> GSGGGDDMSNAGDFLNDNAVEIPSFSKGIINDDEDDEDLMMASGRPRQRSHILEDDENSVDISMLKTGSSLLKEEEEDGQEGSIHNLPLVTSQRPFYDGPMPTPRQKPFQSGSTPLHLTHRFMVWNSIGIIRCYNDEQDNAIDVEFHDTSIHHATHLSNTLNYTIADLSHEAILLACESTDELASKLHCLHFSSWDSSKEWIIDLPQNEDIEAICLGQGWAAAATSALLLRLFTIGGVQKEVFSLAGPVVSMAGHGE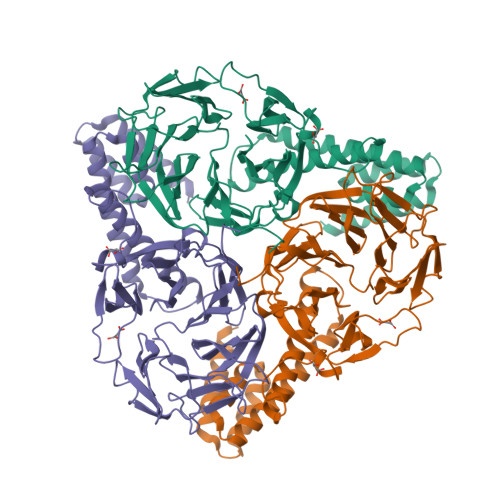QLFIVYHRGTGFDGDQCLGVQLLELGKKKKQILHGDPLPLTRKSYLAWIGFSAEGTPCYVDSEGIVRMLNRGLGNTWTPICNTREHCKGKSDHYWVVGIHENPQQLRCIPCKGSRFPPTLPRPAVAILSFKLPYCQIATEKGQMEEQFWRSVIFHNHLDYLAKNGYEYEESTKNQATKEQQELLMKMLALSCKLEREFRCVELADLMTQNAVNLAIKYASRSRKLILAQKLSELAVEKAAELTAT>MSRIVNVKLSLKRYEYEKPFHITGSVSSESRNVEVEIVLESGVKGYGEASPSFRVNGERVEALLAIENAVREMITGIDVRNYARIFEITDRLFGFPSLKAAVQFATLDALSQELGTQVCYLLGGKRDEIETDKTVGIDTVENRVKEAKKIFEEGFRVIKIKVGENLKEDIEAVEEIAKVTRGAKYIVDANMGYTQKEAVEFARAVYQKGIDIAVYEQPVRREDIEGLKFVRFHSPFPVAADESARTKFDVMRLVKEEAVDYVNIKLMKSGISDALAIVEIAESSGLKLMIGCMGESSLGINQSVH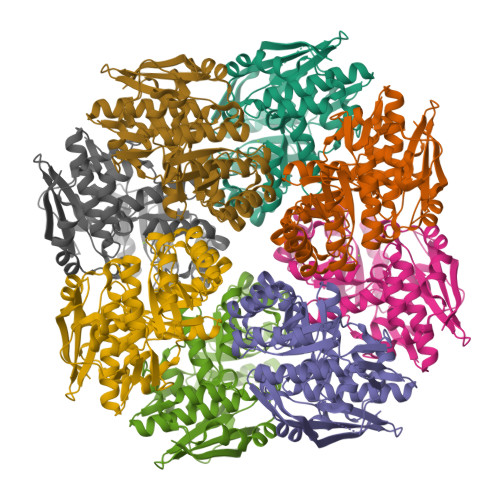FALGTGAFEFHDLDSHLMLKEEVFRGKFIQDGPRMRVKDQ[16x]> HRFRVCALGAAFCVARRWRSGGGPGDRRVRTDWYRCYPSLMEEKDRDMYHCYYPYLFDHGDKMSLYPKIPDNPREWQVEQLQTTYDAIREDKYDAFVRLRAKFPELYQDTYAWDNPPPFGEFNMFYSVRFGMIGVKAFTCKDYDDLGNQFDCTAFWFPDNQIVKHSTRNGDVGTDKVYVGAMNVPVEFHKPHVAAFYKAAGVPVKHVSAGFPVTPDAYAPVGTKLDVRHFKPGQEVTITFQNTDYGYQGVMFRHGFDGGYVWLGDSKWQRRPGCMGAEGQKRIYPGHRMAGQTGASAETYDGVPVWRIDYKNSLIYLPTLIDADVGTYVKFRDTINTKGYTLWNEHRGTPPFPTFIPSEEEDLSKLATDEGQLTSPPLYMYFRDEFAAAQ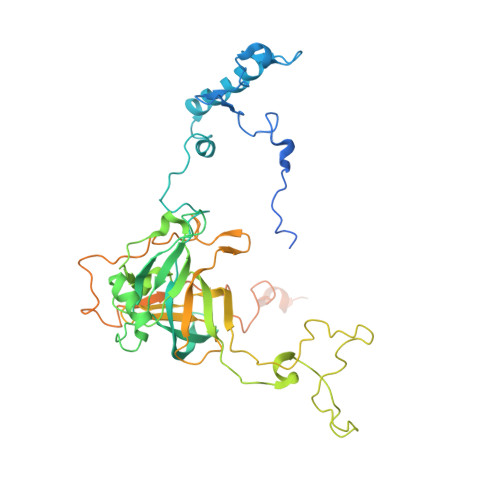LVTQADVEDAKSAKPATAAPKKKVYDLKKYTEARKKYRKNLQKARKYKLMGVRTRAHEKQQEARRAKILKYKRVKT(4~{S})-2-oxidanylidene-4-propyl-pentanedioic acid | C8 H12 O5 | 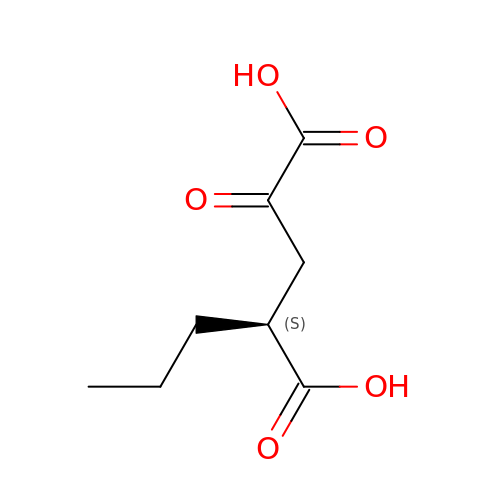UDAAPTAXECGGON-YFKPBYRVSA-N> GKLSEQLKHCNGILKELLSKKHAAYAWPFYKPVDASALGLHDYHDIIKHPMDLSTVKR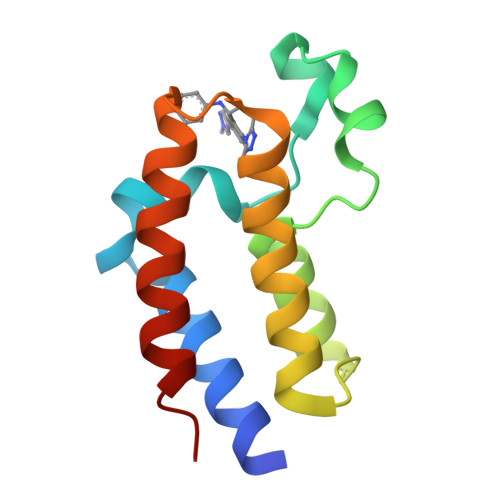KMENRDYRDAQEFAADVRLMFSNCYKYNPPDHDVVAMARKLQDVFEFRYAKMPD>[2x]M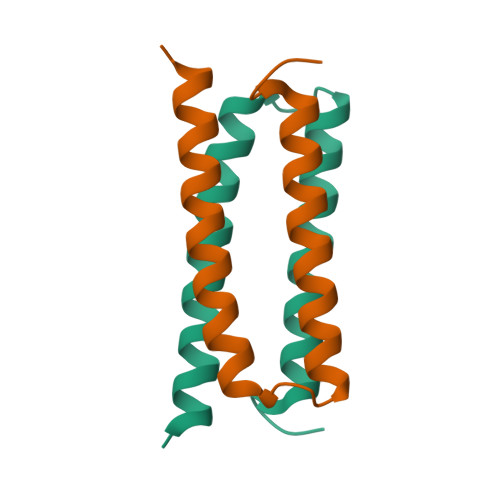SQLGDLGSGAGKGGGGGGSIREAGGAFGKLEAAREEEYFYRKQKEQLERLKNDQIHQAEFHHQQIKEHEEAIQRHKKFLENLTKHHHHHH>[8x]MMVISEKVRKALNDQLNREIYSSYLYLSMATYFDAEGFKGFAHWMKKQAQEELTHAMKFYEYIYERGGRVELEAIEKPPSNWNGIKDAFEAALKHEEFVTQSI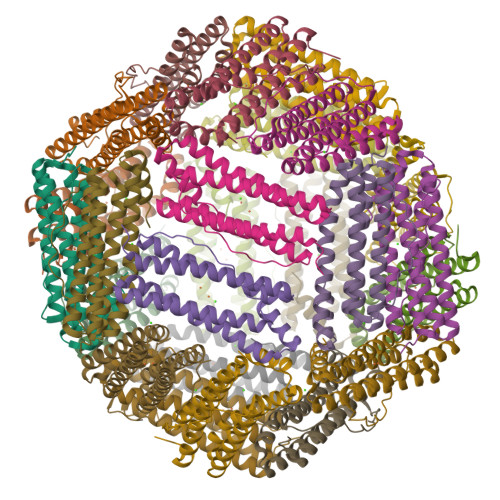YNILELASEEKDHATVSFLKWFVDEQVEEEDQVREILDLLEKANGQMSVIFQLDRYLGQRE>MISLADLQRRIETGELSPNAAIAQSHAAIEAREKEVHAFVRHDKSARAQASGPLRGIAVGIKDIIDTANMPTEMGSEIYRGWQPRSDAPVVMMLKRAGATIIGKTTTTAFASRDPTATLNPHNTGHSPGGSSSGSAAAVGAGMIPLALGTQTGGSVIRPAAYCGTAAIKPSFRMLPTVGVKCYSWALDTVGLFGARAEDLARGLLAMTGRSEFSGIVPAKAPRIGVVRQEFAGAVEPAAEQGLQAAIKAAERAGASVQAIDLPEAVHEAWRIHPIIQDFEAHRALAWEFSEHHDEIAPMLRASLDATVGLTPKEYDEARRIGRRGRRELGEVFEGVDVLLTYSAPGTAPAKALASTGDPRYNRLWTLMGNPCVNVPVLKVGGLPIGVQVIAR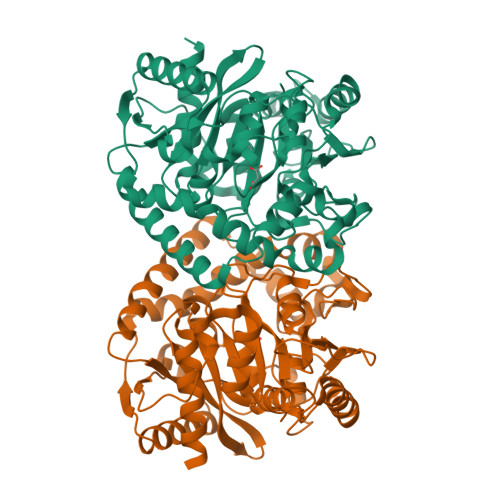FGNDAHALATAWFLEDALAK[2x]> QLHKDPTLDHHWHLWKKTYGKQYKEKNEEAVRRLIWEKNLKFVMLHNLEHSMGMHSYDLGMNHLGDMTSEEVMSLMSSLRVPSQWQRNITYKSNPNRILPDSVDWREKGCVTEVKYQGSCGAAWAFSAVGALEAQLKLKTGKLVSLSAQNLVDCSTEKYGNKGCNGGFMTTAFQYIIDNKGIDSDASYPYKAMDQKCQYDSKYRAATCSKYTE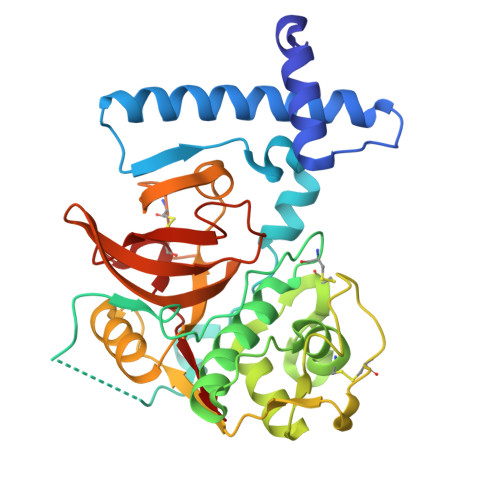LPYGREDVLKEAVANKGPVSVGVDARHPSFFLYRSGVYYEPSCTQNVNHGVLVVGYGDLNGKEYWLVKNSWGHNFGEEGYIRMARNKGNHCGIASFPSYPEI>[2x]NDKLVELSKSDDNWVMPGKNYDSNNFSDLKQINKGNVKQLRPAWTFSTGLLNGHEGAPLVVDGKMYIHTSFPNNTFALGLDDPGTILWQDKPKQNPAARAVACCDLVNRGLAYWPGDGKTPALILKTQLDGNVAALNAETGETVWKVENSDIKVGSTLTIAPYVVKDKVIIGSSGAELGVRGYLTAYDVKTGEQVWRAYATGPDKDLLLASDFNIKNPHYGQKGLGTGTWEGDAWKIGGGTNWGWYAYDPGTNLIYFGTGNPAPWNETMRPGDNKWTMTIFGRDADTGEAKFGYQKTPHDEWDYAGVNVMMLSEQKDKDGKARKLLTHPDRNGIVYTLDRTDGALVSANKLDDTVNVFKSVDLKTGQPVRDPEYGTRMDHLA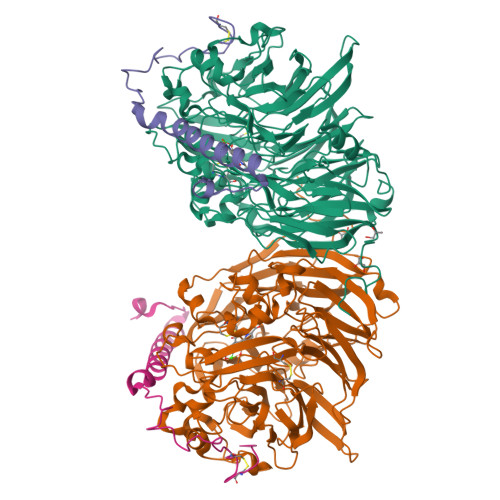KDICPSAMGYHNQGHDSYDPKRELFFMGINHICMDWEPFMLPYKAGQFFVGATLNMYPGPKGDRQNYEGLGQIKAYNAITGDYKWEKMERFAVWGGTMATAGDLVFYGTLDGYLKARDSDTGDLLWKFKIPSGAIGYPMTYTHKGTQYVAIYYGVGGWPGVGLVFDLADPTAGLGAVGAFKKLANYTQMGGGVVVFSLDGKGPYDDPNVGEWKSAAK;>[2x]YDGTKCKAAGNCWEPKPGFPEKIAGSKYDPKHDPKELNKQADSIKQMEERNKKRVENFKKTGKFEYDVAKISAN> GVTKNNSCKKVGVEELINEKGCDLMIIRINRCRGHCFSFTFPNPLTKKYSVHAKCCRM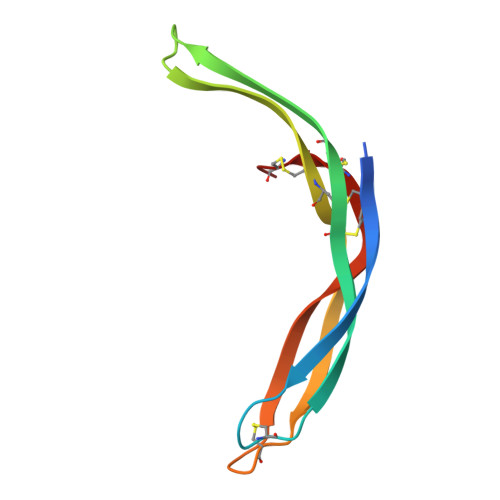VEWEMLETELKCSKGNRNLRIPSATQCECFDCLV>ALLPILSFPDPRLRTIAKPVEEVTDEIRQLAADMFETMYAAPGIGLAASQVDRHIQLIVMDLSESKDEPMVFINPKVTPLTEETQPYEEGCLSVPQIYDKV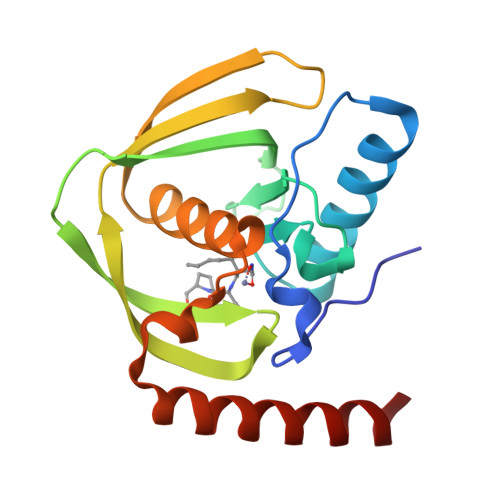DRPSRVKIEAINLEGQAFEIEADGLLAVCIQHEMDHLNGKLFVDYLSPLKRQRAREKVEKIVRQREREKV[2x]thiophene-3-carboxylic 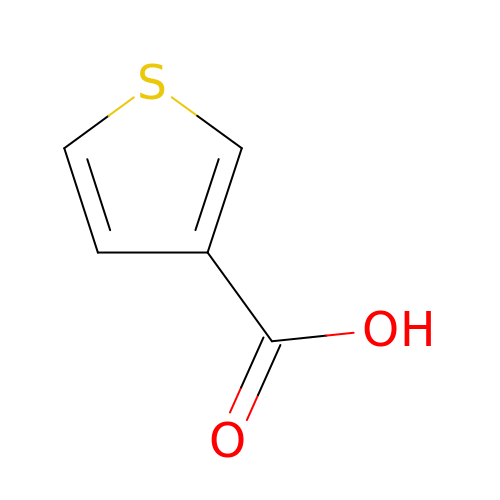acid | C5 H4 O2 S | YNVOMSDITJMNET-UHFFFAOYSA-N In the current study, perdeuterated Pyrococcus furiosus rubredoxin was produced with the iron atom from the [Fe-4S] cluster replaced by the 113Cd isotope. Here we show that it is possible to use neutron anomalous scattering to phase protein crystal structures in a practical fashion. The present demonstration takes advantage of the neutron anomalous scattering properties of 113Cd, the availability of modern high-intensity monochromatic neutron beamlines such as D19 at the ILL, and protein perdeuteration to determine the structure of a biological macromolecule using de novo phasing in a reasonable timescale.

In the current study the anomalous scatterer was introduced in the metal chelating site using chemical reagents to remove the native iron prior to isomorphous replacement with the 113Cd isotope. As pointed out by Bacon19, isotopic replacement of hydrogen by deuterium atoms in a crystal provides a crucial advantage in all but eliminating hydrogen incoherent scattering and thus enhancing the visibility of the anomalous signal. It should be noted that this method may provide a useful complement to X-ray anomalous phasing approaches – particularly where structure determination at room or physiological temperature is advantageous. Anomalous protein phasing work using X-rays can be delicate when carried out at room temperature, and neutron approaches, for which radiation damage effects are essentially negligible, provide a way of tackling these problems. Experiments close to physiological temperatures can highlight structural differences induced by cryo-cooling, and which may be more representative of in vivo structures and their resulting functionalities.

> MAKWVCKICGYIYDEDAGDPDNGISPGTKFEELPDDWVCPICGAPKSEFEKLED The bile acid-sensitive ion channel (BASIC) is the least understood member of the mammalian epithelial Na+ channel/degenerin (ENaC/DEG) superfamily of ion channels, which are involved in a variety of physiological processes. There is, however, a conserved architecture among other members of the ENaC/DEG superfamily. These trimeric channels resemble a chalice in which a large extracellular domain (ECD) connects to a slender transmembrane domain (TMD) via linkers at the membrane interface. In this study, we used single-particle cryo-EM to determine the structure of hBASIC in the membrane-like environment of lipid nanodiscs, confirming its global adherence to the canonical ASIC fold. By determining structures in the presence and absence of Ca2+, we identified a single Ca2+-bound, non-conducting conformation of hBASIC, as well as both conducting and non-conducting conformations of Ca2+-free BASIC, revealing unexpected Ca2+-dependent conformational changes.

To reveal how hBASIC responds to Ca2+ removal, we prepared grids of hBASIC reconstituted in nanodiscs in the presence of 2 mM EGTA to chelate ambient Ca2+o and analyzed the sample using single-particle cryo-EM. The overall resolution of both classes was lower than hBASIC in the presence of Ca2+, with both class 1 and class 2 having a global resolution of ~3.4 Å. In accordance with the electrophysiology data, we observed two distinct particle classes that differ in their pore conformations, which we thus refer to as ‘EGTA-closed’ (class 1), representing a non-conducting state, and ‘EGTA-open’ (class 2), representing an expanded, conducting state. In hBASIC, Ca2+ removal induces a rotation of TM1 and TM2a away from the three-fold axis, resulting in a 4 Å helical displacement of TM1 and a 6° rotation of TM2a. EGTA-closed resembles the Ca2+-closed conformation whereas EGTA-open is dramatically reorientated such that the positions of the L425 and N426 side chains are switched; N426 now facing the vestibule and L425 making contacts with the β1-β2 linker. This is reminiscent of the conformation seen in the MitTx-bound open structure of cASIC1a41. Removal of Ca2+ triggers a 4 Å lateral displacement of the β1-β2 linker, repositioning the tyrosine residue and promoting rearrangement of the β11-β12 linker to open the pore. Removal of Ca2+ leads to rotation of the TM2 helix, displacing these residues from the center of the pore and expanding the extracellular vestibule. The gate is significantly widened in the EGTA-open structure, having a pore radius greater than 2 Å, which is sufficient to accommodate partially dehydrated Na+ ions. Removal of Ca2+ causes rearrangement of this loop to displace the histidine and increase the pore-radius from ~1 Å to ~3 Å.

>FDHDFAISTSFHGIHNIVQNRSKIRRVLWLVVVLGSVSLVTWQIYIRLLNYFTWPTTTSIEVQYVEKMEFPAVTFCNLNRFQTDAVAKFGVIFFLWHIVSKVLHLQEITANSTGSREATDFAASHQNFSIVEFIRNKGFYLNNSTLLDCEFFGKPCSPKDFAHVFTEYGNCFTFNHGETLQAKRKVSVSGRGLSLLFNVNQEAFTDNPALGFVDAGIIFVIHSPKKVPQFDGLGLLSPVGMHARVTIRQVKTVHQEYPWGECNPNIKLQNFSSYSTSGCLKECKAQHIKKQCGCVPFLLPGYGIECDLQKYFSCVSPVLDHIEFKDLCTVGTHNSSCPVSCEEIEYPATISYSSFPSQKALKYLSKKLNQSRKYIRENLVKIEINYSDLNYKITQQQKAVSVSELLADLGGQLGLFCGASLITIIEIIEYLFTNF[3x]>MCTGLRFTDEQGNLYFGRNLDVGQDYGEGVIITPRHYPLPYKFLDNTTTKKAVIGMGIVVDGYPSYFDCYNEDGLGIAGLNFPHFAKFSDGPIDGKINLASYEIMLWVTQNFTHVSEVKEALKNVNLVNEAINSSFAVAPLHWIISDSDEAIIVEVSKQYGMKVFEDKLGVLTNSPDFNWHLTNLGNYTGLNPHDATAQSWNGQKVAPWGVGTGSLGLPGDSIPADRFVKAAYLNANYPAAKGEKANVAKFFNILKSVAMIKGSVVNVQGKDEYTVYTACYSSGSKTYYCNFEDDFELKTYKLDDKTMNSTSLITYHHHHHH[4x]

Bile salt hydrolases (BSHs) comprise a diverse family of microbial enzymes that catalyse critical BA transformation. Primary conjugated BAs synthesized in the liver, such as the tauro- and glycoconjugates of cholic acid (TCA, GCA), are deconjugated by BSHs to generate cholic acid (CA) (BA names and abbreviations are summarized in Supplementary Fig. 1). We found that Lactobacillaceae BSHs display a clear bias for either glycine or taurine-conjugated BAs. Notably, each monomer contains a loop that swaps into the active site of a neighbouring monomer within the tetramer and places amino acids proximal to the catalytic residues.

To examine the molecular foundations of BSH substrate specificity, we determined the crystal structures of six of the Lactobacillaceae BSHs examined above: four glycine-preferring (LgasBSHb, LaciBSHa, LingBSH, LreuBSH) and two taurine-preferring (LgasBSHa, LjohBSHc) BSHs. We examined the sequences of these loops and found that taurine-preferring enzymes exclusively contained G-V/T-G (‘G-X-G’) motifs, while glycine-preferring enzymes solely contained S-R-G/S (‘S-R-X’) motifs. Furthermore, the taurine-preferring LaviBSH, LjohBSHc and LgasBSHa (corresponding to the clusters arrafinosis, johnsonii_1 and gasseri_1, respectively) enzymes are all present within a single major clade, while the LsalBSH (cluster salivarius_1) stands alone in a distantly related branch. This suggests that taurine preference may have evolved twice within Lactobacillaceae. To examine the recalcitrance of MCBAs more broadly, we monitored the deconjugation kinetics of 5 BSHs that had previously exhibited assorted substrate preferences (LingBSH, LgasBSHa, LgasBSHb, LjohBSHc and LreuBSH).> IFKIVQSRLMSTSYHLNSTLES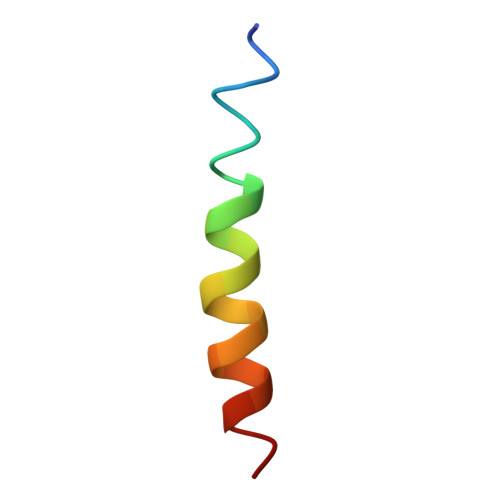LYD> MRRLAFLVVAFCLAVGCFFSPVSKAEGVMSGGDGDKVAVGKDGMVATAHPLASKIGAEVLKKGGNAIDAAIAIQYALNVTEPMMSGIGGGGFMMVYDGETKETSIINSRERAPEGAKPDMFLDEDGKVIPFSERSRHGNAVGVPGTLKGLEAAHKKWGTKKMEDLISPSIKLTEEGFPIDSVLADAIKDHQDKLSKTAAKDIFLPDGEPLKEGDILVQKDMAKT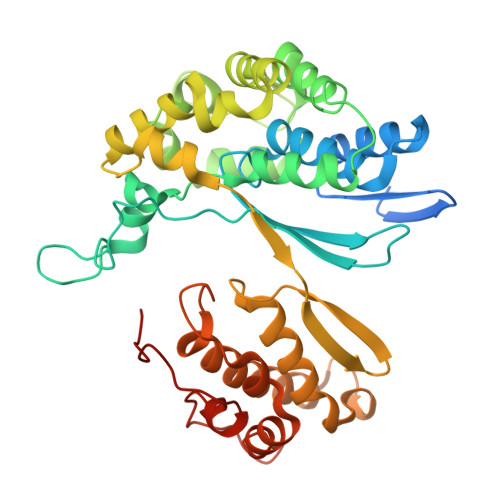FKLIRKEGSKAFYDGEIGRAIADVVQDFGGSMTPDDLSRYEVTTDKPIWGEYHGYDIASMPPPSSGGVFMLQMLKLIDDFHLSQYDPKSFEKYHLLAETMHLSYADRAAYAGDPEFVDVPLRGLLDPDYIKERQKLISLDSMNRDVKEGDPWKYEEGEPNYEIVPQPEDKTIGE>MKELVEIAVPENLVGAILGKG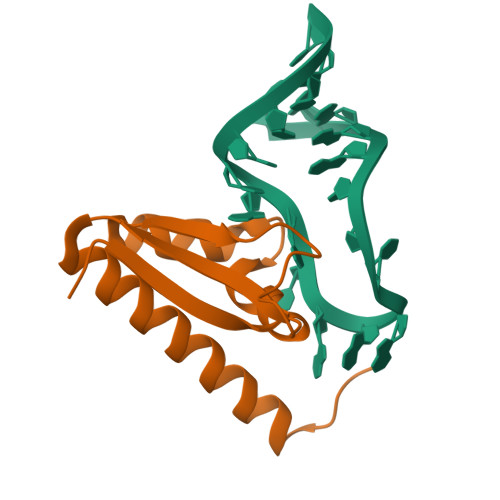GKTLVEYQELTGARIQISKKGEFLPGTRNRRVTITGSPAATQAAQYLISQRVTYEQGVRASNPQKV[2x]> GAMDRLRAAEHPRPDYVLLHISDTHLIGGDRRLYGAVDADDRLGELLEQLNQSGLRPDAIVFTGDLAAKGEPAAYRKLRGLVEPFAAQLGAELVWVMGNHDDRAELRKFLLDEAPSMAPLDRVCMIDGLRIIVLDTSVPGHHHGEIRASQLGWLAEELATPAPDGTILALHHPPIPSVLDMAVTVELRDQAALGRVLRGTDVRAILAGHLHYSTNATFVGIPVSVASATCYTQ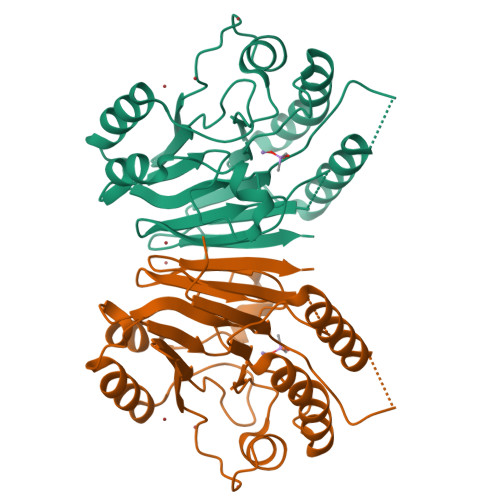DLTVAAGGTRGRDGAQGCNLVHVYPDTVVHSVIPLGGGETVGTFVSP5'-O-[(S)-hydroxy{[(S)-hydroxy(phosphonooxy)phosphoryl]amino}phosphoryl]uridine 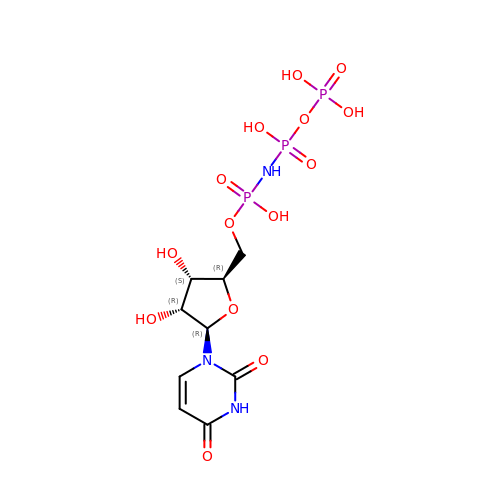| C9 H16 N3 O14 P3 | OZIBFYOFLVBDIY-XVFCMESISA-N>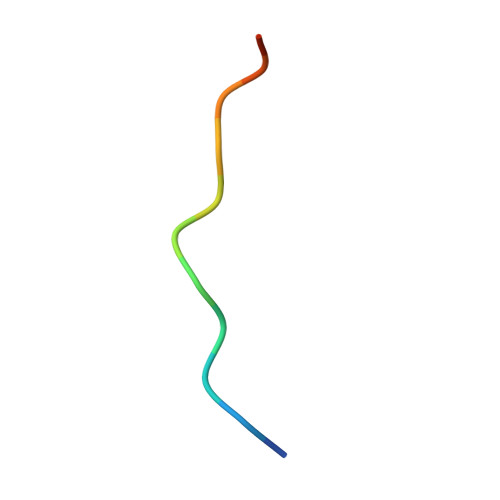 PPPTLPKPKLPKH> SSDRPRGRDPVNPEKLLVITVATAETEGYLRFLRSAEFFNYTVRTLGLGEEWRGGDVARTVGGGQKVRWLKKEMEKYADREDMIIMFVDSYDVILAGSPTELLKKFVQSGSRLLFSAESFCWPEWGLAEQYPEVGTGKRFLNSGGFIGFATTIHQIVRQWKYKDDDDDQLFYTRLYLDPGLREKLSLNLDHKSRIFQNLNGALDEVVLKFDRNRVRIRNVAYDTLPIVVHGNGPTKLQLNYLGNYVPNGWTPEGGCGFCNQDRRTLPGGQPPPRVFLAVFVEQPTPFLPRFLQRLLLLDYPPDRVTLFLHNNEVFHEPHIADSWPQLQDHFSAVKLVGPEEALSPGEARDMAMDLCRQDPECEFYFSLDADAVLTNLQTLRILIEENRKVIAPMLSRHGKLWSNFWGALSPDEYYARSEDYVELVQRKRVGVWNVPYISQAYVIRGDTLRMELPQRDVFSGSDTDPDMAFCKSFRDKGIFLHLSNQHEFGRLLATSRYDTEHLHPDLWQIFDNPVDWKEQYIHENYSRALEGEGIVEQPCPDVYWFPLLSEQMCDELVAEMEHYGQWSGGRHEDSRLAGGYENVPTVDIHMKQVGYEDQWLQLLRTYVGPMTESLFPGYHTKARAVMNFVVRYRPDEQPSLRPHHDSSTFTLNVALNHKGLDYEGGGCRFLRYDCVISSPRKGWALLHPGRLTHYHEGLPTTWGTRYIMVSFVDPAAA

LH3 is therefore a multifunctional enzyme capable of converting collagen lysines into 1,2-glucosylgalactosyl-5-hydroxylysines through three consecutive reactions: hydroxylation of collagen lysines (LH activity), N-linked conjugation of galactose to hydroxylysines (GT activity), and conjugation of glucose to galactosyl-5-hydroxylysines (GGT activity). Here, we present the crystal structures of multifunctional full-length human LH3 in complex with various cofactors and donor substrates. The LH3 monomer encompasses three domains aligned along one direction.

Among these, a very flexible surface loop comprising residues Gly72 to Gly87 is not visible in the electron density of ligand-free LH3 structures. Two tryptophan residues Trp145 and Trp148 proximate to the UDP-binding cavity consistently change their side chain conformations in structures with bound donor substrates. In the absence of donor substrates this residue partially obstructs the cavity, thus acting as a gating residue to host the UDP-glycan. All our LH3 structures systematically showed Fe2+ and 2-OG in the electron density near the core of this domain, confirming that these cofactors are tightly bound to the enzyme and providing a possible explanation for the observed substrate uncoupled LH enzymatic activity. In human LH3, the Fe2+ ion is stabilized by interactions with residue His719 and with residues His667 and Asp669, which constitute part of a HxD motif fully conserved in the Fe2+, 2-OG dioxygenase enzyme family. Residues Tyr656, Cys691 and Arg729 are fully conserved among LH isoforms and delimit the pocket hosting the 2-OG cofactor. In particular, the side chain of free Cys691 contributes to the positioning of the carboxyl moiety of the 2-OG cofactor in the direction of Arg729, forming a salt bridge with the guanidinium group of this residue. Residues 590–610 constitute a flexible loop capping the LH catalytic site.> MRRGALSLLKAGLLGHYQQEAFEARKRFEESTTYPGPIRAATPGDTRFYSGSLESILHDTDRHYWRAVTDDPRVQ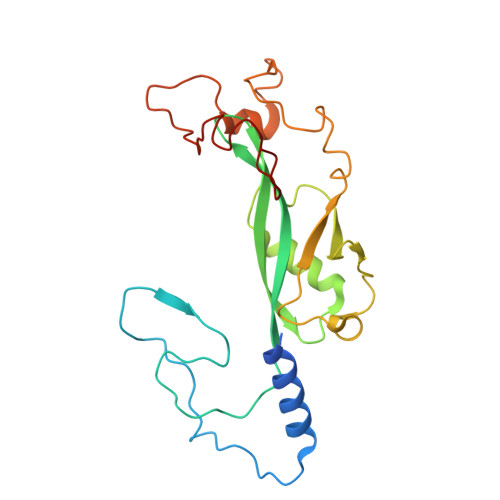HLIPLRIRFKIFTWVTSGWEQRMQVVQIMAPKDSTIAQVKDLVIVENQSPYLCVSSFHLAIDGKELDPQKTLGEYGITEQSQIDAIEQNDHLLHRDDERPRDWTVDEITAEDVKRSPYKEMEMQPLQNLAPRYEARPKGYFGRTYYSGMKQSS>MVMAGASSLDEIRQAQRADGPAGILAIGTANPENHVLQAEYPDYYFRITNSEHMTDLKEKFKRICDKSTIRKRHMHLTEEFLKENPHMCAYMAPSLDTRQDIVVVEVPKLGKEAAVKAIKEWGQPKSKITHVVFCTTSGVDMPGADYQLTKLLGLRPSVKRLMMYQQGCSAGATVLRIAKDLAENNRGARVLVVCSEITAVTFRGPSDTHLDGLVGAALFSDGAAALIVGSDPDTSVGEKPIFEMVSAAQTILPDSDGAIDGHLREVGLVFHL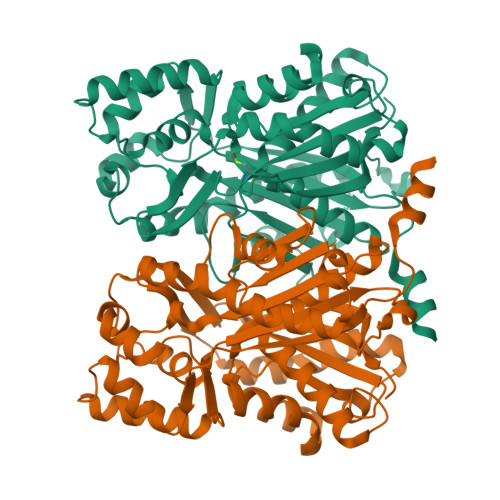LKDVPGLISKNIVKSLDEAFKPLGISDWNSLFWIAHPGGPAILDQVEIKLGLKEEKMRATRHVLSEYGNMSSASVLFILDEMRRKSAKDGVATTGEGLEWGVLFGFGPGLTVETVVLHSVPL[2x]In this article we describe the crystal structure of TarS, an enzyme responsible for the glycosylation of wall teichoic acid polymers of the S. aureus cell wall, a process that has been shown to be specifically responsible for methicillin resistance in MRSA. TarS possesses a catalytic domain with a canonical GTA fold (one of two distinct A/B folds characteristic of nucleotide-sugar dependent glycosyltransferases) consisting of two closely associated α/β/α sandwich Rossmann motifs that abut and form a continuous central β-sheet. TarS possesses a D(91)XDD motif with aspartates coordinating a metal cation, a feature that is typical of the GTA superfamily. Altogether, TarS features a novel architecture with closely-associated trimerization domains connected by a linker region to three protruding catalytic domains that face away from each other.

Brief soaking of the TarS1-349 crystals with UDP-GlcNAc resulted in an enzyme-donor complex with UDP-GlcNAc trapped in the active site as evidenced by the ligand mFo-dFc simulated annealing omit electron density. Our analysis of the enzymatic mechanism of TarS was facilitated by the capture of various TarS1-349 structures encapsulating the catalytic domain in complex with metal and substrates. These include the native structure with bound Mn2+ (free enzyme), the UDP-GlcNAc bound structure in the presence and absence of Mn2+ (the binary Michaelis complex), and the UDP bound structure with Mn2+ (product complex). The first loop, designated as the catalytic site (CS) loop, contains the putative base catalyst D178 and moves towards the catalytic center in the presence of the intact UDP-GlcNAc donor substrate. The second loop, designated as the substrate access (SA) loop, is ordered only in the presence of UDP-GlcNAc and sterically occludes an otherwise open channel leading into the active site in the absence of the intact donor. Notably the side chain carboxylate oxygen of E177, located in the SA loop, moves into position to form hydrogen bonds with the C4 and C6 GlcNAc hydroxyls, the side chain imidazole of H210 and hydroxyl of S212, located in the CS loop, form stabilizing interactions with the O1B and O2B phosphates when ordered upon UDP-GlcNAc binding, and the uracil ring of UDP-GlcNAc is stabilized by offset π-π interactions with the Y10 phenol side chain. Interestingly, no stabilizing interactions are observed with the N-acetyl group of GlcNAc, such that specificity may extend to similar sugars and may be of interest for inhibitor design. UDP-GlcNAc itself is furthermore observed to assume a “tucked under” conformation (as common in other glycosyltransferases), where the GlcNAc sugar is tucked below the plane of the UDP diphosphates, allowing exposure of the scissile bond to nucleophilic attack. The catalytic domain of TarS reveals interesting structural features, such as a CS loop that positions towards the catalytic center and a SA loop that becomes ordered upon donor substrate binding.

>[2x]MKFSVIVPTYNSEKYITELLNSLAKQDFPKTEFEVVVVDDCSTDQTLQIVEKYRNKLNLKVSQLETNSGGPGKPRNVALKQAEGEFVLFVDSDDYINKETLKDAAAFIDEHHSDVLLIKMKGVNGRGVPQSMFKETAPEVTLLNSRIIYTLSPTKIYRTALLKDNDIYFPEELKSAEDQLFTMKAYLNANRISVLSDKAYYYATKREGEHMSSAYVSPEDFYEVMRLIAVEILNADLEEAHKDQILAEFLNRHFSFSRTNGFSLKVKLEEQPQWINALGDFIQAVPERVDALVMSKLRPLLHYARAKDIDNYRTVEESYRQGQYYRFDIVDGKLNIQFNEGEPYFEGIDKLVPRGSAAAALEHHHHHH>GSHMATPWSGYLDDVSAKFDTGVDNLQTQVTEALDKLAAKPSDPALLAAYQSKLSEYNLYRNAQSNTVKVFKDIDAAIIQNFRGGSGGTTISDAEIWDMVSQNISAIGDSYLGVYENVVAVYTDFYQAFSDILSKMGGWLLPGKDGNTVKLDVTSLKNDLNSLVNKYNQINSNTVLFPAQSGSGVKVATEAEARQWLSELNLPNSCLKSYGSGYVVTVDLTPLQKMVQDIDGLGAPGKDSKLEMDNAKYQAWQSGFKAQEENMKTTLQTLTQKYSNANSLYDNLVKVLSSTISSSLETAKSFLQG[2x]

Bacterial infections including Salmonellosis and Shigellosis affect millions of people every year. These bacteria use a T3SS to secrete virulence factors to manipulate host cells. The T3SS is a multi-component system that forms a continuous protein transport channel through the two bacterial membranes and the periplasmatic space that extends into the surrounding medium by a needle structure. Tip proteins, which bind to the distal end of the T3SS needle, are thought to play an important role in this process. SipD from S. typhimurium, IpaD from Shigella flexneri and BipD from Burkholderia mallei are tip proteins that are thought to interact with their corresponding needle subunits PrgI, MxiH and BsaL, respectively, to make the needle tip complex.

Here, we address the questions of how the Salmonella SipD interacts with PrgI and deoxycholate and the mechanistic consequences of the assembly of the T3SS needle tip complex. We could show that two different proteins, structurally conserved in many pathogenic bacteria, bind each other to constitute the needle tip of the transport system. Bile salts influence the T3SS of intestinal bacteria. For instance, the presence of deoxycholate either impedes (S. typhimurium) or facilitates (S. flexneri) host invasion. Noteworthy, it was recently shown that SipD and IpaD bind deoxycholate and some of its derivatives.>[2x]EPTRIATNDRLSAAVCFDALVFLSGQVPGQAEDIHGQTR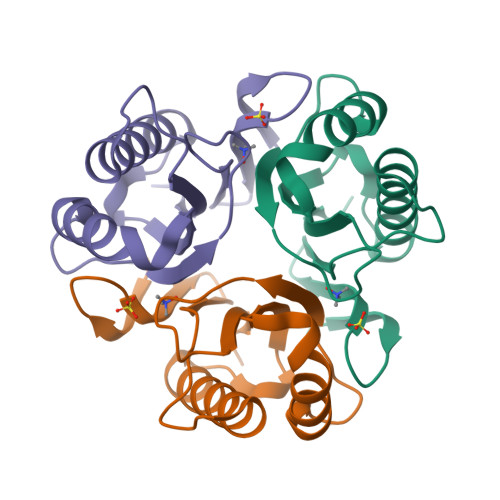EVLAKIDALLAEAGSRKERILSATIYLKDIARDFAALNEVWTQWLPTGQAPSRTTVQAELARPSVLVEITVVAARG> 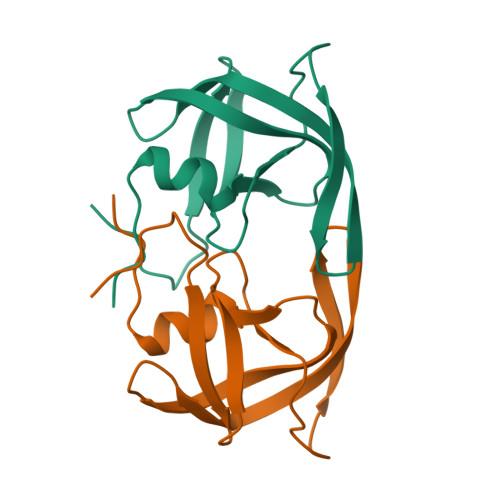PQFSLWRRPVVTAHIEGQPVEVLLDTGADDSIVTGIELGPHYTPKIVGGIGGFINTKEYKNVEIEVLGKRIRGTIMTGDTPINIFGRNLLTALGMSLNF>[3x]MISILHYGYSFIMLLGALYFYLLSKDPKGVPASEYLIAMVIPLWSGAAYLSIALGQGLFQYDDTTIYYARYIDWVISTPLLLAALAL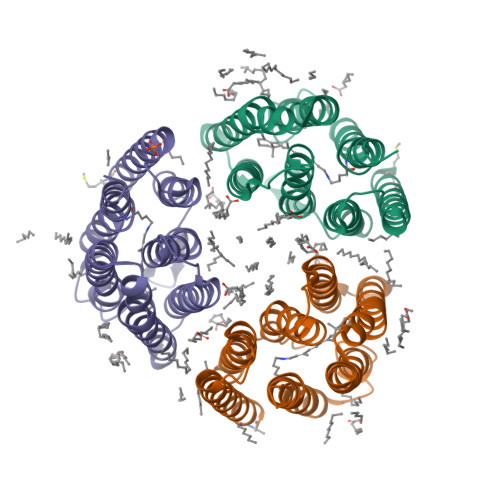TAMFGGKKNLTLLFSLVALDVFMIITGFVADLSIGTTKYIWYSLGVIALIIILVITFGPLRRIALSNGTRLARHYTRVAIYLSALWVCYPTAWLLGPSGLGLAQELTEVLVFIILPIFSKVGFSIVDLHGLRKLHQSSYVHNA>[2x]MNHKVHHHHHHMELGTLEGSMAGARCRTLYPFSGERHSQGLRFSAGELLTLLQVPDGGWWEGEKDDGLRGWFPASYVQLLEKPGMVPPPPGEESQTVILPPGWHSYLSPQGRRYYVNTTTNETTWERPSSSPGISASPGPHRSSLPTTVNGYHASGTPAHPPETAHMSLRKSTGDSQNLGSSSPGRKQSKENTITINCVTFPHPDTMPEQQLLKPTEWSYCDYFWADKKDPQGNGTVAGFELLLQKQLKGKQMQKEMSEFIRERIKIEEEYAKNLAKLSQNSLAAQEEGSLGEAWAQVKKSLADEAEVHLKFSAKLHSEVEKPLMNFRENFKKDMKKCDHHIADLRKQLASRYASVEKARKALTERQKDLEMKTQQLEIKLSNKTEEDIKKARRKSTQAGDDLMRCVDLYNQAQSKWFEEMVTTTLELERLEVERVEMIRQHLCQYTQLRHETDMFNQSTVEPVDQLLRKVDPAKDRELWVREHKTGNIRPVDMEI

In this study, we show that GAS7 plays a critical role in phagocytic cup formation in macrophages. Crystallographic, electron microscopic, biochemical and cellular localization analyses revealed that the GAS7 F-BAR domain possesses unique hydrophilic loops that contribute to two-dimensional sheet formation of GAS7 on flat membranes of phagocytotic cup, indicating that the sheet-like assembly of GAS7 is essential for phagocytosis. In addition to the F-BAR domain, GAS7b possess a WW domain, and GAS7cb and GAS7c possesses a WW and an SH3 domain, while GAS7d contains only the F-BAR domain. The structures of the F-BAR domains in both crystals were almost identical, with a root mean square deviation of 1.2 Å. The GAS7 F-BAR domain forms a helical-bundle dimer with a shallow concave curvature, which is one of the flattest curvatures amongst the known F-BAR domains.

GAS7b (Mus musculus and Homo sapiens), GAS7cb (Mus musculus), and GAS7c (Homo sapiens) are GAS7 splicing isoforms. To understand the functions of GAS7, we determined the crystal structure of the GAS7 F-BAR domain, using the crystals of an F-BAR fragment and GAS7cb. In the crystals of GAS7cb, only the F-BAR domain was visible in the electron density maps. In the GAS7cb crystals, the periodicity observed on the monolayered membrane appeared to be absent. The monolayers showed the striations formed by the GAS7 F-BAR domain, GAS7b and GAS7cb, all of which indicated the sheet-like GAS7 assemblies with striations similar to each other on the membrane. The zymosan phagocytosis was rescued by the endogenous-level forced expression of GAS7b and GAS7cb in the knockout cells, but not by the GAS7b ΔFFL2 mutant or the F-BAR domain fragments.TRANS-(1S,2S)-2-AMINO-1,2,3,4-TETRAHYDRONAPHTHALEN-1-OL | C10 H13 N O | 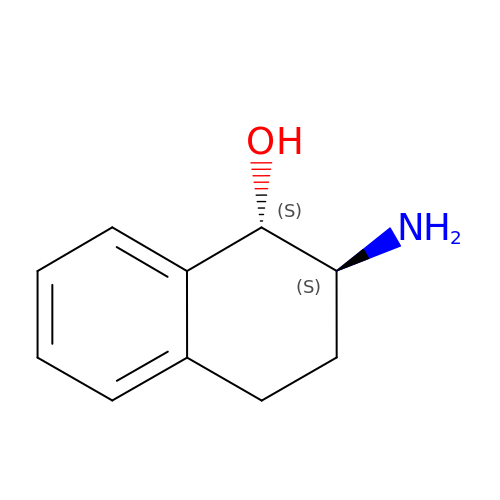IIMSEFZOOYSTDO-UWVGGRQHSA-N> MRIGIISVGPGNIMNLYRGVKRASENFEDVSIELVESPRNDLYDLLFIPGVGHFGEGMRRLRENDLID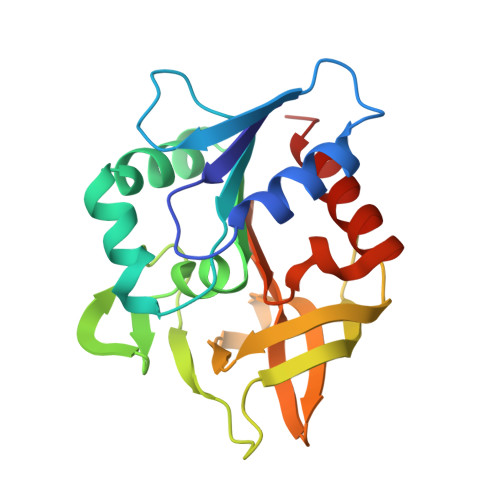FVRKHVEDERYVVGVCLGMQLLFEESEEAPGVKGLSLIEGNVVKLRSRRLPHMGWNEVIFKDTFPNGYYYFVHTYRAVCEEEHVLGTTEYDGEIFPSAVRKGRILGFQFHPEKSSKIGRKLLEKVIECSLSRR While most SAM riboswitches strongly discriminate between SAM and SAH, the SAM/SAH riboswitch responds to both ligands with similar apparent affinities. The riboswitch forms an H-type pseudoknot structure with coaxial alignment of the stem–loop helix (P1) and the pseudoknot helix (PK). An additional three base pairs form at the non-open end of P1, and the ligand is bound at the interface between the P1 extension and the PK helix. Binding SAM or SAH stabilizes the PK helix, so structuring the Shine–Dalgarno sequence, sequestering it and preventing initiation of translation (OFF state).

The structure of the riboswitch bound to SAM was solved by SAD using the anomalous scatter of the bromine, and the other complexes were solved by molecular replacement using that structure. The majority were solved in C2, giving six crystallographically-independent molecules for each. In the C2 crystal lattice, six rod-like riboswitch molecules associate in the form of a triangle in the crystal lattice. The edges of the triangle are formed by coaxial stacking of the P1 helices of two RNA molecules, and the vertices of the triangle are formed by a crossing of the PK helices at 60°. The structures were unaffected by crystal contacts: the structure of the riboswitch bound to SAM was solved in space groups P312 and C2, with an all-atom RMSD of 0.26 Å. The importance of these contacts for ligand binding have been explored using atomic mutagenesis and isothermal titration calorimetry (ITC). Both SAH and SAM resulted in exothermic binding of ligand with closely similar calculated affinities of Kd = 20 and 19 μM respectively. Electron density for the remaining part of the methionine is not visible for the bound SAM ligand, but is observable for the bound dCSAH showing that the primary amine is hydrogen bonded to U23 O4 just as it is for SAH. The sulfur atom is 3.8 Å away from the nearest RNA atom, leaving enough space to accommodate the SAM methyl group without steric clash, and the open binding site will readily accommodate the trajectory of the chain with a planar thioether (SAH) or tetrahedral sulfonium (SAM). In addition there is no electrostatic interaction with the positively charged sulfonium ion as there is in the SAM-II and V riboswitches. The structure therefore explains why this riboswitch binds both SAM and SAH with similar affinities.

>GGUCACAACGGCUUCCUGGCGUGACC[6x];>AUUGGAGCA[6x]> MHHHHHHSQQLQLRVQGKEKHQTLEVSL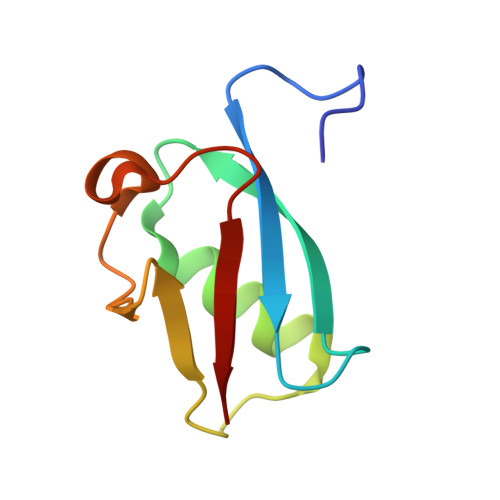SRDSPLKTLMSHYEEAMGLSGRKLSFFFDGTKLSGRELPADLGMESGDLIEVWG> AQKTFKVT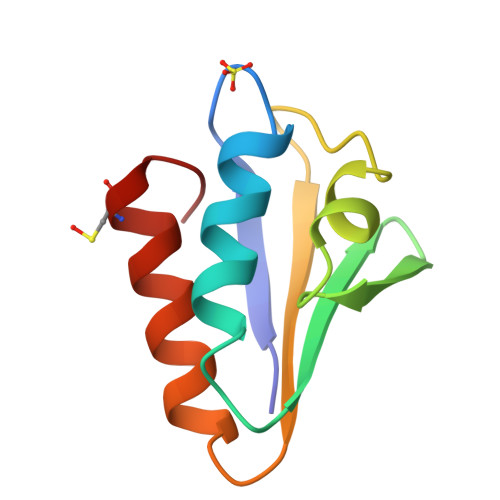ADSGIHARPATVLVQTASKYDADVNLEYNGKTVNLKSIMGVVSLGIAKGAEITISASGADENDALNALEETMKCEGLGE6-{[4-(trifluoromethyl)phenyl]methyl}-2H-1,3-benzodioxol-5-ol | C15 H11 F3 O3 | 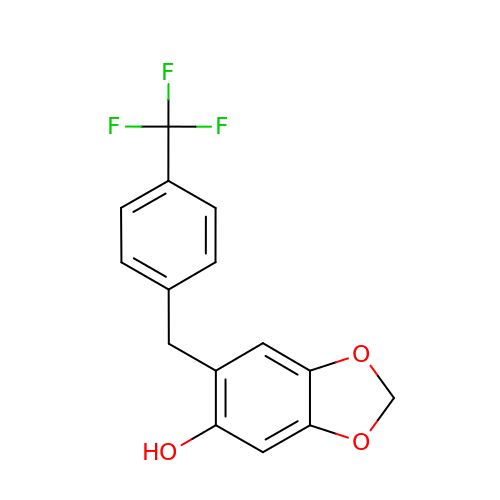CZTARKWMYGFNTE-UHFFFAOYSA-N(2~{R})-1-[4-(4-ethanoyl-3-ethyl-5-methyl-1~{H}-pyrrol-2-yl)-1,3-thiazol-2-yl]-~{N}-[3,3,3-tris(fluoranyl)propyl]piperazine-2-carboxamide 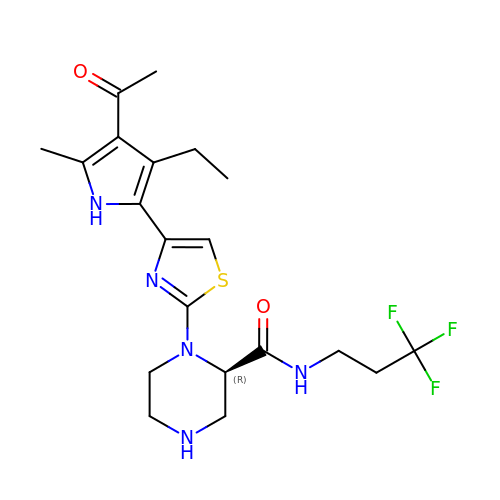| C20 H26 F3 N5 O2 S | PLKCLYWKGAEBFY-OAHLLOKOSA-N>[4x]MDQKPQPAKTHATEVTVLEGK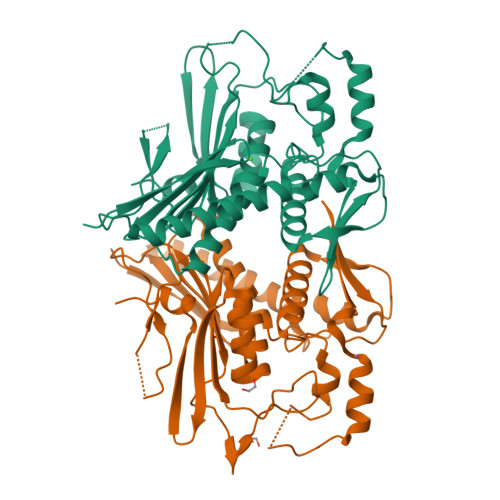TMGTFWRASIPGIDAKRSAELKEKIQTQLDADDQLLSTYKKDSALMRFNDSQSLSPWPVSEAMADIVTTSLRIGAKTDGAMDITVGPLVNLWGFGPEQQPVQIPSQEQIDAMKAKTGLQHLTVINQSHQQYLQKDLPDLYVDLSTVGKGYAADHLARLMEQEGISRYLVSVGGALNSRGMNGEGLPWRVAIQKPTDKENAVQAVVDINGHGISTSGSYRNYYELDGKRLSHVIDPQTGRPIEHNLVSVTVIAPTALEADAWDTGLMVLGPEKAKEVVRREGLAVYMITKEGDSFKTWMSPQFKSFLVSEKNLEHHHHHH>MIAELFTNNALNLVIIFGSCAALILMSFWFRRGNRKRKGFLFHAVQFLIYTIIISAVGSIINYVIENYKLKFITPGVIDFICTSLIAVILTIKLFLLINQFEKQQIKKGRDITSARIMSRIIKITIIVVLVLLYGEHFGMSLSGLLTFGGIGGLAVGMAGKDILSNFFSGIMLYFDRPFSIGDWIRSPDRNIEGTVAEIGWRITKITTFDNRPLYVPNSLFSSISVENPGRMTNRRITTTIGLRYEDAAKVGVIVEAVREMLKNHPAIDQRQTLLVYFNQFADSSLNIMVYCFTKTTVWAEWLAAQQDVYLKIIDIVQSHGADFAFPSQTLYMDNITPPEQGRHHHHHH[7x]

Mechanosensitive channel of small conductance (MscS) has an indispensable role in the protection of bacterial cells when the cells experience a transfer from a high osmolarity medium to a low osmolarity environment. In the present study, we characterize a Na+/K+ cation-selective MS channel, YnaI, which exhibits small conductance among the family of MS channels in E. coli.

To understand the molecular mechanism of the Na+/K+-selective characterization of YnaI, we solved its structure at an overall resolution of 3.8 Å (3.6 Å at the cytoplasmic domain) by cryo-EM single-particle method. Similar to previously reported MscS structures, YnaI comprises seven YnaI promoters bearing the MscS channel fold and forming a homoheptamer. The heptamer extends ~117 Å parallel to the sevenfold axis, with ~87 Å in width in the perpendicular direction. Secondary structure analysis predicts that YnaI contains five TM helices, while we only identified two transmembrane helices (TMH4 and TMH5) in each YnaI protomer, which may be due to the flexibility of the other three TMHs. Consistent with other MscS channels, YnaI contains a large cytoplasmic domain and comprises the middle β-domain, α/β domain, and a C-terminal extension forming an interior chamber of about 30 Å in diameter. The isolated C-terminus of β10 in each monomer forms a seven-stranded parallel β-barrel (residues 327–343), leading to the formation of a potential channel pore (referred to as the β-barrel pore hereafter). The structure of YnaI closely resembles that of the closed conformation of TtMscS and EcMscS with root-mean-square deviations (rmsd) of 3.05 Å and 2.3 Å over 223 Cα atoms of the overall structures, respectively. These structural observations suggest that YnaI structure was resolved at a non-conducting state. Indeed, YnaIM158A in the TM region alters the mean reversal potential from −39.2 ± 0.5 mV to −20 ± 0.5 mV, corresponding to decreased cation-to-anion (PK:PCl) permeability ratio from 9:1 to 3:1. Further simulation and mutagenesis validation supported that seven methionine residues formed a circle and bound anions with different binding energy, leading to elegant modulation of further passing of cations.> GKKRQWALEDFEIGRPLGKGKFGNVYLAREKQSKFILALKVLFKAQLEKAGVEHQLRREVEIQSHLRHPNILRLYGYFHDATRVYLILEYAPLGTVYRELQKLSKFDEQRTATYITELANALSYCHSKRVIHRDIKPENLLLGSAGELKIADFGWSCHAPSSRRTTLSGTLDYLPPEMIEGRMHDEKVDLWSLGVLCYEFLVGKPPFEANTYQETYKRISRVEFTFPDFVTEGARDLISRLLKHNPSQRPMLREVLEHPWITANSS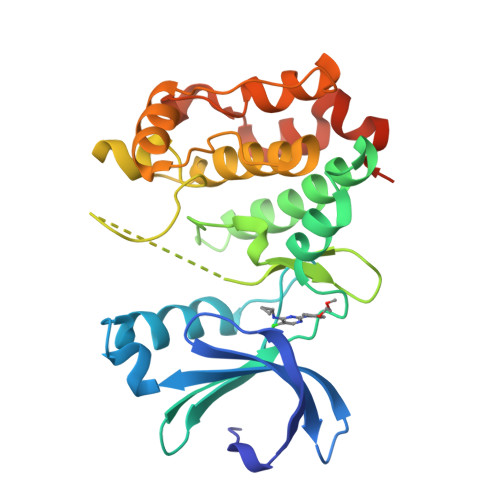KPSNSQNKESASKQS> MSQSTASLVPEGNQGSLQEDVSFDFNGVPGQALDAVRMRLAQLTHSLRRIRDEMSKAELPQWYTLQSQLNVTLSQLVSVTSTLQHFQETLDSTVVYPLPKFPTTSHESLVTTLLRKKNIPEVDEWMKYVRETSGVTTALLKDEEIEKLLQQDREITNWARTTFRNEYGKHDFKNEESLSEEHASLLVRDSKP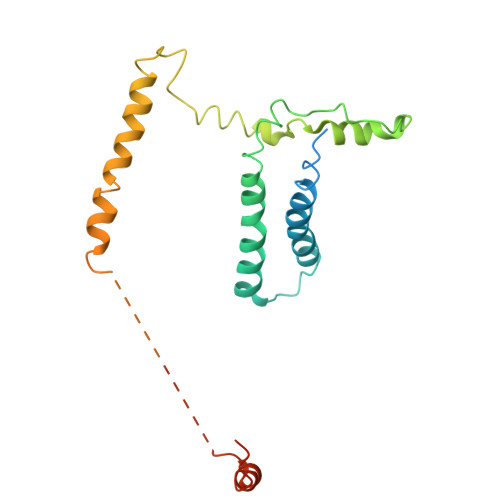SKPFNVDDVLKFTFTGEKPIITGSTSTSSSN> GPGSMSETVSDWVPTGAVTVRAPGKVNLYLAVGDLRDDGYHELTTVFHAVSLADDVTVRDADVLSIDVVGQGEGTVPTDERNLAWQAA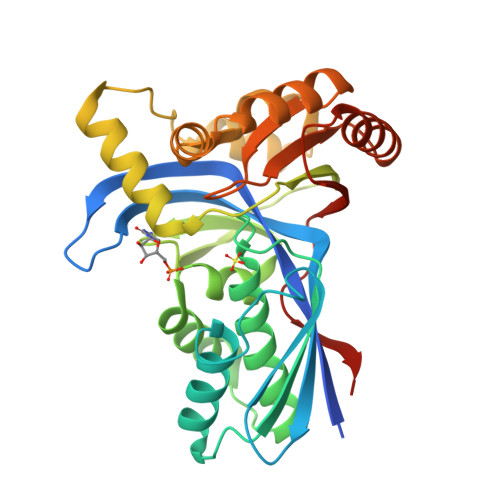ELFADHVGRAPDVSIFINKDIPVAGGMAGGSADAAAVLVAMNELWHAGVPRRDLHHLAAQLGSDVPFALHGGTALGTGRGEQLATVLARNVFHWVFAFADGGLATPQVFKEIDRLRENGDPPRLAEADELLGALAAGDARRLAPLLGNELQAAAVSLNPELRRTLRAGESAGALAGIVSGSGPTCAFLCTSADDAVQVSAELAGAGVCRTVRVASGPVHGAQVIQGRSDG ISPINESIB MESILATE | 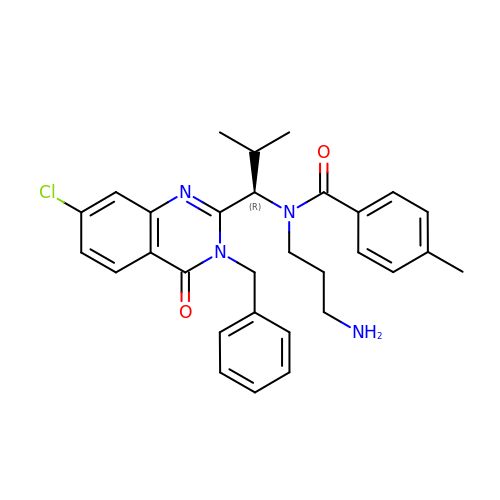C30 H33 Cl N4 O2 | QJZRFPJCWMNVAV-HHHXNRCGSA-N>GAMDAKRSAEALVPRFQFERLLNQDQAGRRSALYGAIDGQPALLILERAPFPTSTAYLGRAANTLRALTNLGANDIYHWYL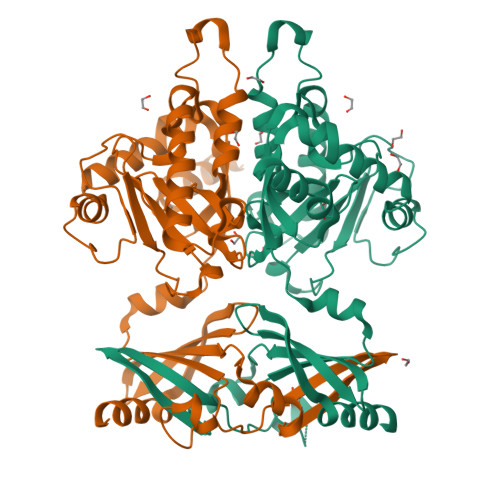ASSGVIEIPVEESEGTDDEFADLKINLIYPCTEKHVKKYSKQGVRFVTETPEIYRDYVRPYMQAQREAGRLNWVYNIIEGRKEVEDVIYRTPYGQDPEEGFLLLPDLNWDRKTVEALHLLGIVERRDLWSLRDLKKKHLPWLRHMREKLIEATTKVYPTVEADQLKLYLHYQPTYYHLNIHIVHVQLEAGATQATGKAVGLESVMEQLEHMHVGPEDGDGSDVGMDRVTMCYTLGEASDLWVDVFEPLKRKKQARPTSEPGAASQSQ[2x]> TP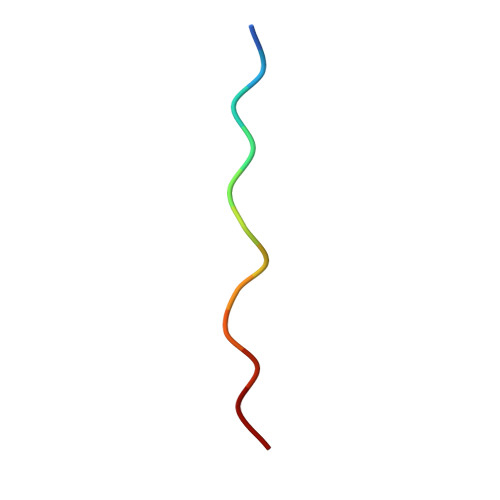TVAPPAPVYR>[9x]MAHIFVKPELVAEIGVKQLQREIVLPGLVWTNPLTDFGGSKNDTITVRVPAITTANRRDLRDPDRTVIASELVEHSFGVTLDKHVYAALKFTDEQRTLDIRDYTKQVLMPQVSAVAYELEDYIAELIEGAPYEETILIDPADTVPAFITADQRMGEANVP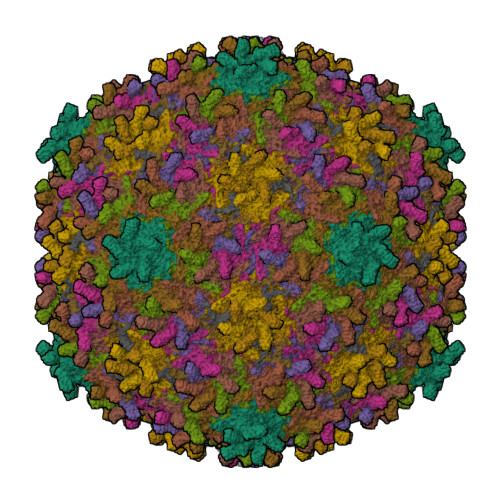TDSRRLVVGSAVAAALAKDKQFRHADWSGDQANAALREAHVGRLAGMNVIRSNAIAPDKAYLWHRTAFILAYRTPVVPEGAKAGASFSANGVALRWLADYDYSQLGDRTLLDVFTGRKVVTEVDGSFVRAVELQLQASSITIVGGAFALATTTGTKQLKVRDDNGTDVTARCTFASSAGTKATVSAAGLVTGVAAGTADITASYVPPQGGTAKTATVTVTVP;>[2x]MGLISDPVEVDPIQVGRDEAGWVQELRDREAWPKQEVPEQAKKPAKVGN(2S,8R,9S,15S)-15-CYCLOHEXYL-9,12-BIS(CYCLOPROPYLMETHYL)-8-HYDROXY-20-METHYL-4,7,11,14,17-PENTAOXO-2-PHENYL-18-OXA-3,6,10,12,13,16-HEXAAZAHENICOSAN-1-OIC 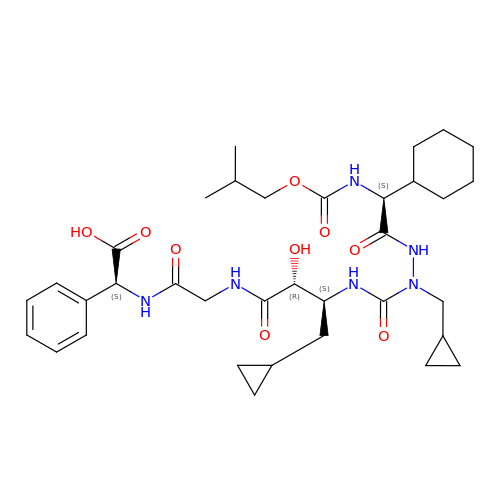ACID | C35 H52 N6 O9 | PLFWZBVXDUFZCY-ZVVXMFRTSA-N>[2x]MKSSFSGKYQLQSQENFEAFMKAIGLPEELIQKGKDIKGVSEIVQNGKHFKFTITAGSKVIQNEXTVGEEAEMETMTGEK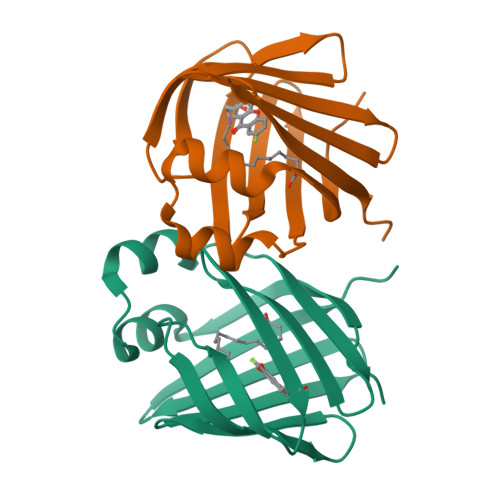VKTVVQLEGDNKLVTTFKNIKSVTELNGDIITNTMTLGDIVFKRISKRILEHHHHHH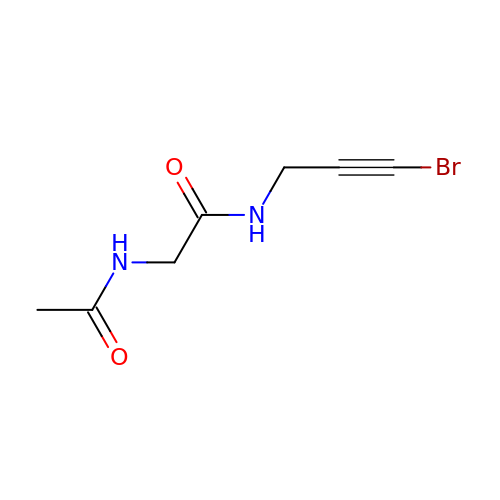2-acetamido-N-(3-bromanylprop-2-ynyl)ethanamide | C7 H9 Br N2 O2 | VNYCHSVZFAMMQB-UHFFFAOYSA-N> ADPKAANLSGLTDAQAKEFHEHWKHGVWSWV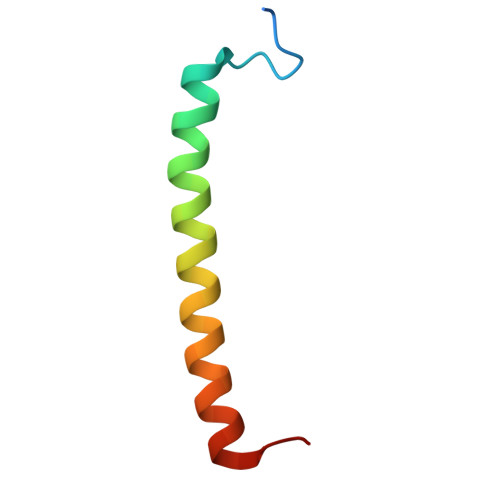MIASAVHVVTWIYQPWF> MKRRWKKNFIAVSAANRFKKISSSGALENLYFQGEMVSVIDKLVFDFGGKTLVS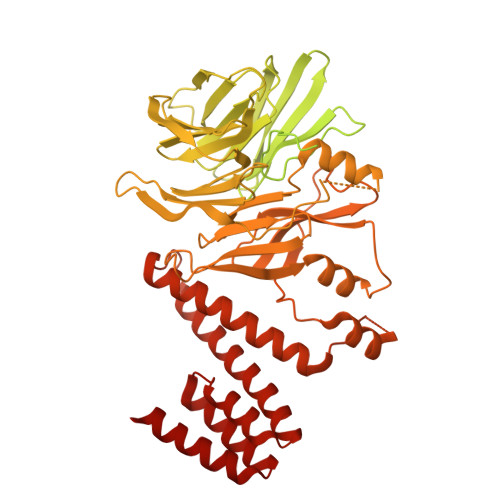LAPDNNTLCVANKNGLTKILKTNNPEEEPETLDSSKLVSSIKCYSNSHFLMTTMQGDALRYNIDSSQEELLARFALPLRDCCVIHSGKMAVFGGDDLELILLELDDETHKKHAIKIDEQVSQISYNSQMNILAVSMINGKVQIFSLTSTIPNKVHELNDYIVANSYDDTHRDKILSNMMDDIDKDNDNDLSETADPDENNVADPEFCAANRICTRVAWHPKGLHFALPCADDTVKIFSIKGYSLQKTLSTNLSSTKAHFIDLQFDPLRGTYIAAVDLNNKLTVWNWETSEIHYTREFKRKITNIAWKIQADSKTLDLVLGTWSGSIAIVQNLAESVVSNIPDQSVAESSTKHGLFVDSESDLENLEGNDDINKSDKLFSDITQEANAEDVFTQTHDGPSGLSEKRKYNFEDEEDFIDDDDGAGYISGKKPHNEHSYSRVHKTHSFPISLANTGKFRYMPFSPAGTPFGFTDRRYLTMNEVGYVSTVKNSEQYSITVSFFDVGRFREYHFEDLFGYDLCFLNEKGTLFGQSKTGQIQYRPHDSIHSNWTKIIPLQAGERITSVAATPVRVIVGTSLGYFRSFNQFGVPFAVEKTSPIVALTAQNYRVFSVHYSQFHGLSYSLSELGTSSKRYYKRECPLPMSLPNINSDMKKDANLDYYNFNPMGIKSLFFSSYGDPCIFGSDNTLLLLSKWRSPEESKWLPILDSNMEIWKMSGGKETTDIHVWPLALAYDTLNCILVKGKHIWPEFPLPLPSEMEIRMPVFVKSKLLEENKAILNKKNEIGADTEAEEGEEDKEIQIPVSMAAEEEYLRSKVLSELLTDTLENDGEMYGNENEVLAALNGAYDKALLRLFASACSDQNVEKALSLAHELKQDRALTAAVKISERAELPSLVKKINNIREARYEQQLK>MHHHHHHENLYFQGHMKKWGDMFTWGVSTSSYQIEGAANQGGRGPSIWDTFSKIPGAVANGDNGDVACDHYHRYNEDLDLMKWLGVGAYRFSIAWPRVIPSGYGALNKEGMDFYDRLIDGALERGITPWPTLYHWDLPQSLQDKGGWNNRDCAYWFAEYSQKMAEAFSDRLKNWITINEPFCSAWLGHLYGVMAPGIKDLKTGINA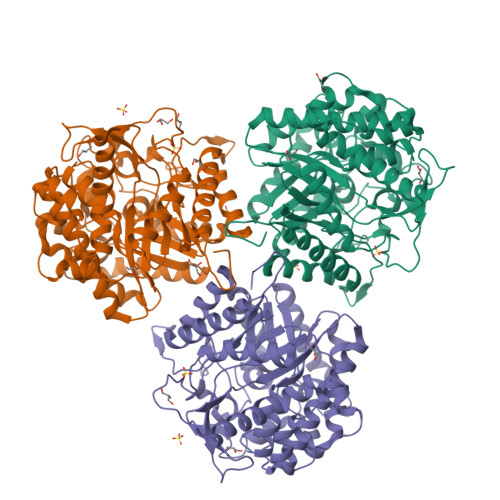SHHLLLGHGLATKAIREVSSELKVGITLNFTPAITLGESSEDKLAVELADGFDNRWFGDPVFKAKYPEDIVKAFGKEVPIHPGDMEIISTPLDYLGLNYYFRQTVEYDATAKPLPYKQVTAPNVERTGMGWEVHAQSFTELLERVSKEYKPKEIFITENGSAWDDEVVDGKVDDPNRVSYLERHLDAMFAAKNKGVPISGYFAWSLIDNFEWAYGYAKRFGIIYVDYQTQKRIPKSSAYYYQKRIKES[3x]>[3x]MGSDKIHHHHHHMFLGEDYLLTNRAAV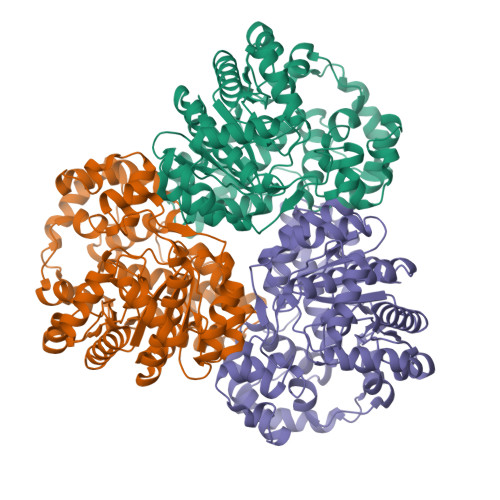RLFNEVKDLPIVDPHNHLDAKDIVENKPWNDIWEVEGATDHYVWELMRRCGVSEEYITGSRSNKEKWLALAKVFPRFVGNPTYEWIHLDLWRRFNIKKVISEETAEEIWEETKKKLPEMTPQKLLRDMKVEILCTTDDPVSTLEHHRKAKEAVEGVTILPTWRPDRAMNVDKEGWREYVEKMGERYGEDTSTLDGFLNALWKSHEHFKEHGCVASDHALLEPSVYYVDENRARAVHEKAFSGEKLTQDEINDYKAFMMVQFGKMNQETNWVTQLHIGALRDYRDSLFKTLGPDSGGDISTNFLRIAEGLRYFLNEFDGKLKIVLYVLDPTHLPTISTIARAFPNVYVGAPWWFNDSPFGMEMHLKYLASVDLLYNLAGMVTDSRKLLSFGSRTEMFRRVLSNVVGEMVEKGQIPIKEARELVKHVSYDGPKALFFG PPLPs are found across apicomplexan species, and contain a conserved central membrane attack complex/perforin (MACPF) domain, as well as a unique C-terminal domain, named the Apicomplexan PLP C-terminal β-pleated sheet (APCβ) domain, and a variable N-terminal domain. The MACPF superfamily represents an ancient homologous group of pore forming proteins, which function principally in cellular attack or defense. PPLP1 is implicated in cell traversal by sporozoites across the mammalian dermis and into the liver to invade hepatocytes and replicate within a parasitophorous vacuole (PV), as well as in the evasion of host phagocytic immune cells. PPLP1 also plays a role in erythrocyte egress by the merozoite stage (gametocyte) of the *Plasmodium* life cycle, via membrane disruption.

The structure of PvPLP1 APCβ domain was determined by X-ray crystallography at 3.15 Å resolution, to reveal as expected three β-stranded repeat motifs arranged in a prism ([Fig fig1]; see [Table tbl1] for data collection and refinement statistics). Each repeat consists of an inner four-stranded β-sheet and an outer two-stranded β-sheet, locked together by two disulfide bonds. Comparison with TgPLP1 APCβ domain (root mean standard deviation, RMSD = 0.978Å between 170 atom pairs) reflects a conserved C-terminal domain architecture across the *Toxoplasma* and *Plasmodium* APCβ domains. Flexible loops between the inner and outer beta-sheets in the third repeat, which are absent in the crystal structure, were subsequently modelled in for molecular dynamics (MD) studies (see [Sec s4] below). Three 100 ns atomistic MD simulations of the PvPLP1 APCβ domain structure indicated that the overall structural core was stable, at an average RMSD of 2.5 Å, while the modelled loops were more flexible. Comparison of loops of APCβ in PvPLP1and TgPLP1 reveals that PvPLP1 lacks an extended loop and any aromatic residues at that point in the structure, containing instead several polar and aliphatic hydrophobic residues, as well as a histidine residue at its end rather than a tryptophan. PvPLP1 did not bind to any mammalian membrane lipid species tested while PvPLP2 recognized anionic lipid species, with a strong preference for phosphatidylinositol 4-phosphate (PI(4)P), followed by palmitoyloleoylphosphatidylserine (PS) and Cardiolipin, and a weak association with the other phosphatidylinositol phosphates (PIPs) ([Fig fig2]). Sets of 20 simulations for each protein were performed. Only two binding events were observed in PvPLP1 simulations ([Fig fig3] and Fig S6). Similar binding energies of −15 and −19 kJ mol^−1^ were obtained for PvPLP2 and TgPLP1 respectively, while the absence of an energy well for PvPLP1 indicates it has no affinity for the PC:PE:PS (45:45:10) bilayer ([Fig fig3]).

>ETGKDIVKILTASTTVTKTGPPPISAECPHNMVVLFGFVVKQNFWDHTNKLQSYEMEICESGASSCTSKQGNTNKYDVSYTYIECGPQALPFTEQVVSVSGTTYNSVKCPNDYSVLFGFGMATSSGRHQSALYSYFTPCRPGLKSCSLNMNEHDDKSYIYLVCVDATIWTGLNALSMIAKDDLHSAVNRYQQFNDGELVVTCPSEGTILTGFYGETHTSSPYVTVPFGKCAKSLKACSVHGSGQAIGIHNYRTLFTVALCKNNKTHHHHHH[2x]>CGIVGIAGVMPVNQSIYDALTVLQHRGQDAAGIITIDANNCFRLRKANGLVSDVFEARHMQRLQGNMGIGHVRYPTAGSSSASEAQPFYVNSPYGITLAHNGNLTNAHELRKKLFEEKRRHINTTSDSEILLNIFASELDNFRHYPLEADNIFAAIAATNRLIRGAYACVAMIIGHGMVAFRDPNGIRPLVLGKRDIDENRTEYMVASESVALDTLGFDFLRDVAPGEAIYITEEGQLFTRQCADNPVSNPCLFEYVYFARPDSFIDKISVYSARVNMGTKLGEKIAREWEDLDIDVVIPIPETSCDIALEIARILGKPYRQGFVKNRYVGRTFIMPGQQLRRKSVRRKLNANRAEFRDKNVLLVDDSIVRGTTSEQIIEMAREAGAKKVYLASAAPEIRFPNVYGIDMPSAT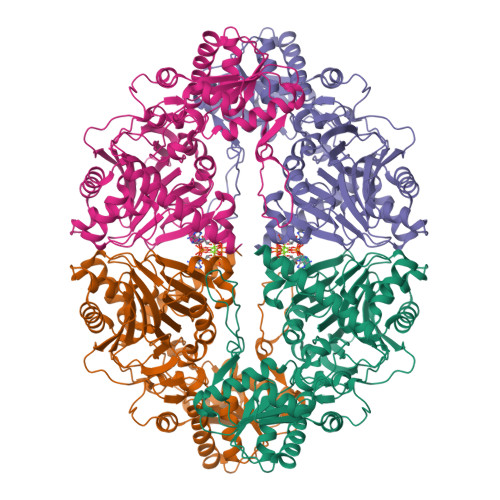ELIAHGREVDEIRQIIGADGLIFQDLNDLIDAVRAENPDIQQFECSVFNGVYVTKDVDQGYLDFLDTLRNDDAKAVQRQNEVENLEMHNEG[2x]>HMCDSALTAQANDLRIYQVMVESFVNGDDAIGHGTGYGTSHHKGDLQGIIDSLDYIESLGMNAIWLTPIFDSIPVEGQDHWADRLDATGYFTSNYFAVDPRFGTMEQAKELVEKAHEKGLYVFFDGVFGHHKDNVVPSPEGRLPVGENNPVSYPESLAFYQEVATFWIEELKIDGWRLDQAYQVPTEAWTAIRASVDEASKSVTYVNSKGEAVNPLGYMVAEIWNNENYIKETGYGAEGEPALCSAFDFPVRYRVVETFAANENGIGNKGGKWLDEGMNLHRLYPSHAQPNLMLGNHDLVRFGDLLQRGNIASPEQAEYWERHKAALSFQAAYSGPITLYYGEEIGDELEGYAQKVEQDCAVQGLCDDHVARTSANIDGLTVNLNEKQRDLKQYVSQLMTLRAAHPALSRGERTNIVANETVYIDHKQADDDALIYMVSTTADQDTVELKASDIASDGQLVDLLTGKVHSAINGEYQISLAPFEAKFLLIETPSASGLTKVATVSAASSLIGEGFMAQCDNPTIEGDGPIGKTLYVVGDFADASWKQKPHRAYRYVGENTYQAVVDEKAGAFRMQYASKDWSPQFTADGLELTPGKTASLKRGGYGQDTAVTLPEAGQYVWSLKFTDSGDPEQIMVSKCP[4x]

The GH13_37 subfamily is the most recently established α-amylase subfamily. It was created on the basis of the isolation and phylogenetic analysis of a novel α-amylase, designated AmyP, from a marine metagenomic library. AmyP exhibits high substrate specificity for starch over pullulan or cyclomaltodextrins, efficiently hydrolyzing starch into glucose, maltose and maltotriose. AmyP is a raw-starch-degrading enzyme (RSDE), thus making it of potential interest in the food processing and green-fuels communities. The AmyPΔSBD is composed of A, B, and C domains and shares structural features with other GH13 α-amylases.

The crystal structure of WT AmyPΔSBD complexed with maltose was obtained through co-crystallization of full-length WT AmyP with β-cyclodextrin (β-CD), an unpreferred substrate of AmyP (AmyP/β-CD). This structure was determined to a resolution of 1.95 Å by using the AmyP-E221Q/γ-CD structure as an initial model. The structure of AmyP-E221Q/γ-CD contains electron density representing a maltotriose molecule bound to the active site and occupying subsites -1, -2 and -3, whereas the structure of AmyP/β-CD contains electron density representing a maltose molecule at subsites -2 and -3. These observations suggested that the E221Q mutant possesses activity for γ-CD and the WT enzyme possesses activity for β-CD at the high concentration in the crystallization drop, thus producing maltotriose from γ-CD and maltose from β-CD, respectively. The maltose bound to the active pocket of the WT enzyme also superimposed well at subsites -2 and -3 with the maltotriose bound to the active site of the E221Q mutant. The observed binding of maltose in subsites -2 and -3 indicated that the affinity of subsite -3 for a glucose residue is greater than that of subsite -1. The observation that G2 binds in subsites -2 and -3 indicates tighter binding in these subsites than in subsite -1, which is consistent with the production of a limit digest of G1, G2 and G3 by the enzyme. It seems likely that a strong -3 subsite would protect G3 from rapid digestion, whereas a weak -1 subsite would limit the formation of glucans smaller than G3. The AmyPΔSBD-E221Q/G3 and AmyPΔSBD/G2 structures can therefore explain the nature of the limit digest of G1, G2 and G3 by the AmyP enzyme.> MRFPSIFTAVLFAASSALAAPVNTTTEDETAQIPAEAVIGYLDLEGDFDVAVLPFSNSTNNGLLFINTTIASIAAKEEGVSLDKREAEAWHWLQLKPGQPMYKREAEAEAWHWLQLKPGQPMYKREADAEAWHWLQLKPGQPMYKREADAEAWHWLQLKPGQPMYXXXXXXXXX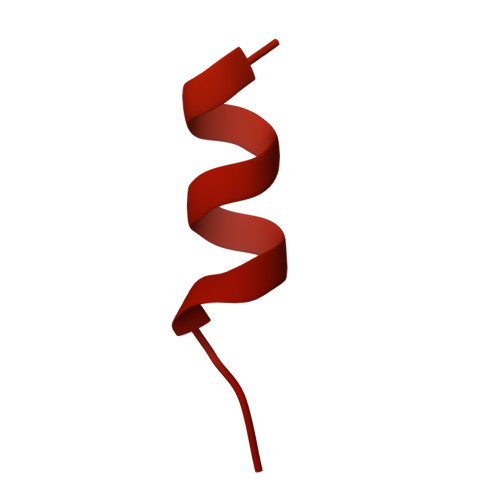XXXX Proteins of the Ras superfamily of small GTPases regulate a variety of cellular processes such as intracellular transport, cell shape and motility, as well as differentiation and growth. For all of these processes, switching between the active GTP-bound and the inactive GDP-bound states is of fundamental importance. We describe here the synthesis of reactive acryl derivatives of guanine nucleotides that are able to react covalently with strategically placed cysteines in GTPases to lock them into their functional states in an irreversible manner. Extensive analysis of biochemical and structural features demonstrate the maintenance of the signalling ability of the modified GTPases.

Extending the labelling experiments to other GTPases, placing a cysteine at the position equivalent to E35 in Rab1b led to covalent interaction with aGTP for all those tested (Rab5A, Rab6A, Rab7A, Rab8A, Ypt7, HRas and Cdc42), albeit at variable rates, but substitution of cysteine at positions corresponding to L125 in Rab1b only led to covalent reaction in the case of Rab7A. In order to determine the structure of the GTP-bound state, we introduced two further mutations in addition to the cysteine at position 35: one of these was Q68L, a position equivalent to the GTP hydrolysis-deficient Rab1Q67L variant. However, Ypt7Q68L hydrolysed GTP faster than Rab1Q67L and we reasoned based on structure and amino acid sequence comparisons that the residue K38Ypt7 (I37 in Rab1) close to the γ-phosphate might play a significant role. We therefore introduced a further change at this position (K38I). Using this Ypt7 variant, we were able to produce a covalently linked aGTP adduct that was stable enough to allow crystallization within 12 h at 4 °C and allowed structure determination. Structural comparison of these adducts with Ypt7:GDP and Ypt7:GppNHp demonstrates that the covalent linker provides sufficient flexibility to allow the covalently locked proteins to adopt similar conformations of the nucleotide-binding pocket and in particular of the switch I region of Ypt7Q35C–aGDP, Ypt7Q35C–aGppNHp and Ypt7Q35C,K38I,Q68L–aGTP compared with the non-covalently nucleotide-bound proteins. Despite this flexibility, the electron density around the nucleotide and the linker was well defined in Ypt7Q35C–aGDP and Ypt7Q35C,K38I,Q68L–aGTP, whereas in Ypt7Q35C–aGppNHp this was only true for two (chains A and B) out of four copies within the asymmetric unit. In conclusion, the structures of Ypt7 modified with aGDP, aGTP or aGppNHp are very similar to the non-covalent Ypt7:nucleotide complexes, demonstrating that the structural properties of GTPases are maintained in covalently modified proteins.

> GHMSSRKKNILKVIILGDSGVGKTSLMHRYVNDKYSCQYIATIGADFLTKEVTVDGDKVATMQVWDTAGLERFQSLGVAFYRGADCCVLVYDVTNASSFENIKSWRDEFLVHANVNSPETFPFVILGNKIDAEESKKIVSEKSAQELAKSLGDIPLFLTSAKNAINVDTAFEEIARSALQQNQA> TAELKICRVNRNSGSCLGGDEIFLLCDKVQKE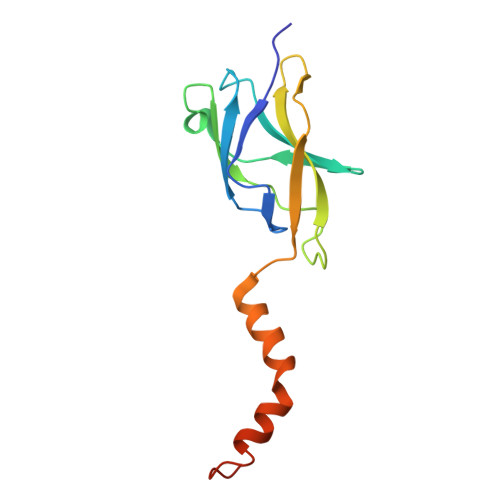DIEVYFTGPGWEARGSFSQADVHRQVAIVFRTPPYADPSLQAPVRVSMQLRRPSDRELSEPMEFQYLPDTDDRHRIEEKRKRTYETFKSIMKKSPFNGPTEPRP> MRFKKHVVQHEETMQAIAQRYYGDVSYWIDLVEHNNLKYPYLVETDEEKMKDPERL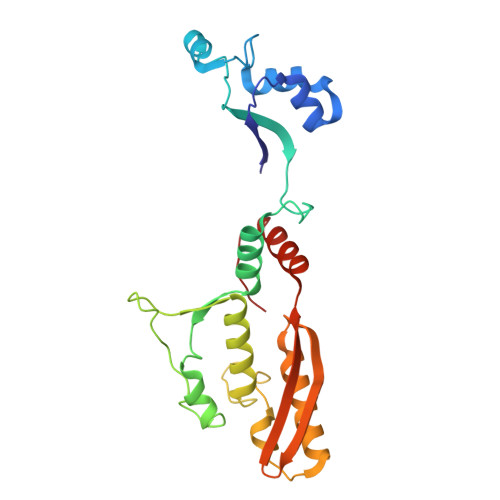ASTGDTLIIPIESDLTDVSAKEINSRDKDVLVELALGRDLNITADEKYFNEHGTSDNILAFSTNGNGDLDTVKGIDNMKQQLQARLLTPRGSLMLHPNYGSDLHNLFGLNIPEQATLIEMEVLRTLTSDNRVKSANLIDWKIQGNVYSGQFSVEIKSVEESINFVLGQDEEGIFALFE> WGNLGHETVAYIAQSFVASSTESFCQNILGDDSTSYLANVATWADTYKYTDAGEFSKPYHFIDAQDNPPQSCGVDYDRDCGSAGCSISAIQNYTNILLESPNGSEALNALKFVVHIIGDIHQPLHDENLEAGGNGIDVTYDGETTNLHHIWDTNMPEEAAGGYSLSVAKTYADLLTERIKTGTYSSKKDSWTDGIDIKDPVSTSMIWAADANTYVCSTVLDDGLAYINSTDLSGEYYDKSQPVFEELIAKAGYRLAAWLDLIASQPS

S1 nuclease from Aspergillus oryzae (EC 3.1.30.1; NCBI sequence ID: XP_001818636; S1–P1 nuclease family in Pfam, PF02265) is an extracellular, single–strand–specific, sugar non–specific, Zn2+–dependent, fungal nuclease with 3'–mononucleotidase activity with a pH optimum in range 4.0–4.3. S1 nuclease has the phospholipase C/P1 nuclease–like fold stabilized by two disulfide bridges. The active site is located in a surface cleft and composed of the obligatory catalytic trinuclear zinc cluster supplemented by Lys68 and the nucleoside binding site 1 (NBS1; also called Phe site in the previous studies). A cluster of three zinc ions coordinates the substrate/product scissile phosphate and the reaction mechanism utilizes water activated by Zn2+ ions as a nucleophile.

A phosphate ion inside the zinc cluster in the first binding mode is modeled with occupancy 0.5. Phosphate ion is a product of 3’–mononucleotidase activity and simultaneously an inhibitor of S1 nuclease. This structure brings evidence for one of its binding modes and for its capability to bind inside the active site. The inhibition effect of inorganic phosphate was tested on ssDNase activity of S1wt under standard reaction conditions. Phosphate inhibits activity by 70% at 10 mM concentration and by 91% at 100 mM concentration.> MASAEVVSKLEAAFAKLQNASDCHSLLKKYLTKEVFDQLKGKQTKMGATLMDVIQSGVENLDSGIGVYAPDAESYTLFAALLDPIIEDYHKGFKPSDKQPPKDSGDLNTFIDVDPDKKYVISTRVRCGRSLEGYPFNPCLKKQQYEEMESRVKGQLESMSGELRGKYYPLTGMTKETQKQLIDDHFLFKEGDRFLQAAHACKFWPTGRGIYHNDAKTFLVWVNEEDHLRIISMQKGGNLKEVFGRLVTAVGVIEEKVKFSRDDRLGFLTFCPTNLGTTIRASVHIKLPKLGADRKKLEEVAAKYNLQVRGTAGEHSDSPDGVYDISNKRRLGLSEY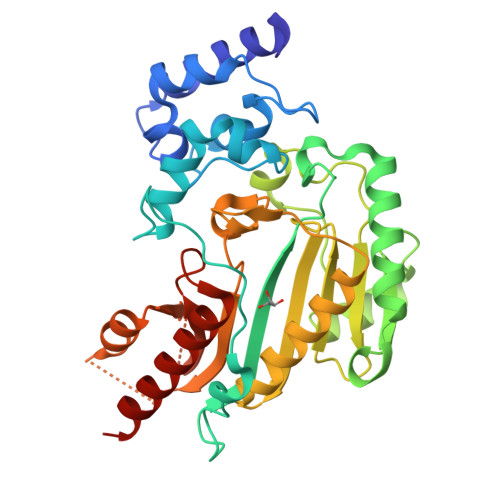EAVKEMQDGILELIKAEESAR>SNAMNYNFNEIVDRSNNFSSKWSEMEKKYGTNDLLPMWVADMDFKAAPCIIDSLKNRLEQEIYGYTTRPDSYNESIVNWLYRRHNWKIKSEWLIYSPGVIPAISLLINELTKANDKIMIQEPVYSPFNSVVKNNNRELIISPLQKLENGNYIMDYEDIENKIKDVKLFILCNPHNPVGRVWTKDELKKLGDICLKHNVKIISDEIHSDIILKKHKHIPMASISKEFEKNTITCMAPTKTFNIAGLQSSYVVLPDEKDYKLLDDAFTRIDIKRNNCFSLVATEASYNNGESWLESFLEYLESNIDFAIKYINENMPKLKVRKPEGTYLLWVDFSALGLSDEELESIL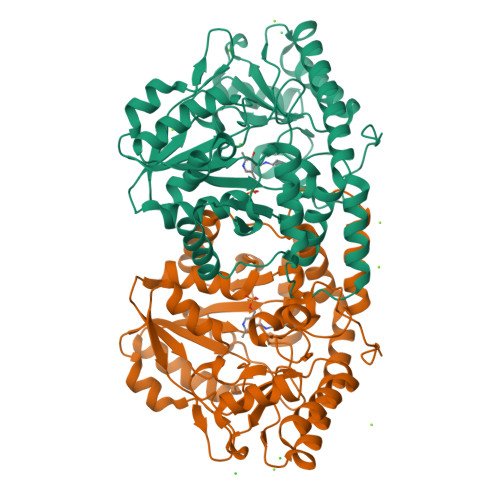VQKGKVALNQGNSFGIGGSGYQRINLACPRSMLEEALIRIKNAIN[2x]(3S,4S)-1-[(2-chlorophenyl)sulfonyl]-N-[(2E)-2-iminoethyl]-4-(morpholin-4-ylcarbonyl)pyrrolidine-3-carboxamide 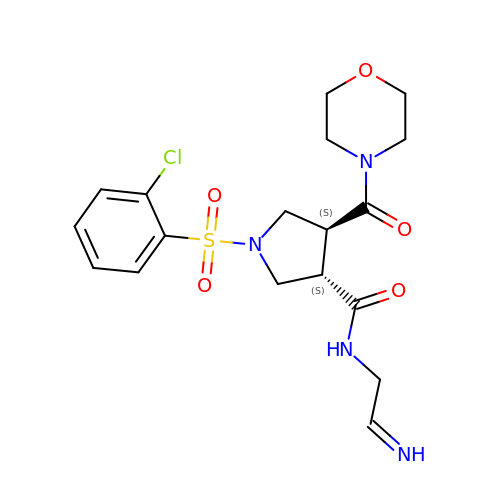| C18 H23 Cl N4 O5 S | PZXUNWUKBPZQOX-HASADGDUSA-N>MGATGDAEQPRGPSGAERGGLELGDAGAAGQLVLTNPWNIMIKHRQVQRRGRRSQMTTSFTDPAISMDLLRAVLQPSINEEIQTVFNKYMKFFQKAALNVRDNVGEEVDAEQLIQEACRSCLEQAKLLFS[4x];>[4x]MAQTQGTRRKVCYYYDGDVGNYYYGQGHPMKPHRIRMTHNLLLNYGLYRKMEIYRPHKANAEEMTKYHSDDYIKFLRSIRPDNMSEYSKQMQRFNVGEDCPVFDGLFEFCQLSTGGSVASAVKLNKQQTDIAVNWAGGLHHAKKSEASGFCYVNDIVLAILELLKYHQRVLYIDIDIHHGDGVEEAFYTTDRVMTVSFHKYGEYFPGTGDLRDIGAGKGKYYAVNYPLRDGIDDESYEAIFKPVMSKVMEMFQPSAVVLQCGSDSLSGDRLGCFNLTIKGHAKCVEFVKSFNLPMLMLGGGGYTIRNVARCWTYETAVALDTEIPNELPYNDYFEYFGPDFKLHISPSNMTNQNTNEYLEKIKQRLFENLRMLPHAPGVQMQAIPEDAIPEESGDEDEDDPDKRISICSSDKRIACEEEFSDSEEEGEGGRKNSSNFKKAKRVKTEDEKEKDPEEKKEVTEEEKTKEEKPEAKGVKEEVKLA;>GAVSIEPRINVGSRFQAEIPLMRDRALAAADPHKADLVWQPWEDLESSREKQRQVEDLLTAACSSIFPGAGTNQELALHCLHESRGDILETLNKLLLKKPLRPHNHPLAT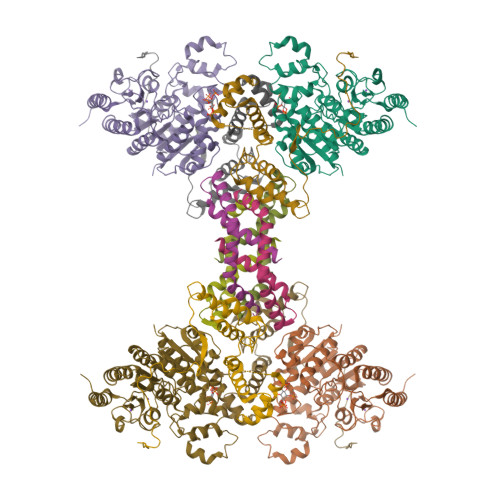YHYTGSDQWKMAERKLFNKGIAIYKKDFFLVQKLIQTKTVAQCVEFYYTYKKQVKIGRNGTLT[4x]>MKFLVNVALVFMVVYISYIYADPSGPPAPRHLHAQALSDSEIQLTWKHPEALPGPISKYVVEVQVAGGAGDPLWIDVDRPEETSTIIRGLNASTRYLFRMRASIQGLGDWSNTVE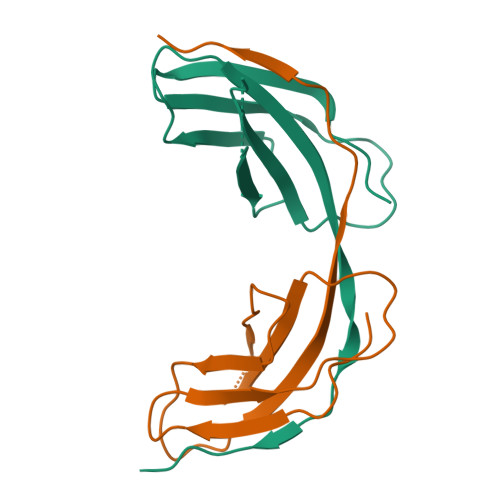ESTLGHHHHHH[2x]> MAIRLYKLAVALGVFIVSAPAFSHGHHSHGKPLTEVEQKAANGVFDDANVQNRTLSDWDGVWQSVYPLLQSGKLDPVFQKKADADKTKTFAEIKDYYHKGYATDIEMIGIEDGIVEFHRNNETTSCKYDYDGYKILTYKSGKKGVRYLFECKDPESKAPKYIQFSDHIIAPRKSSHFHIFMGNDSQQSLLNEMENWPTYYPYQLSSEEVVEE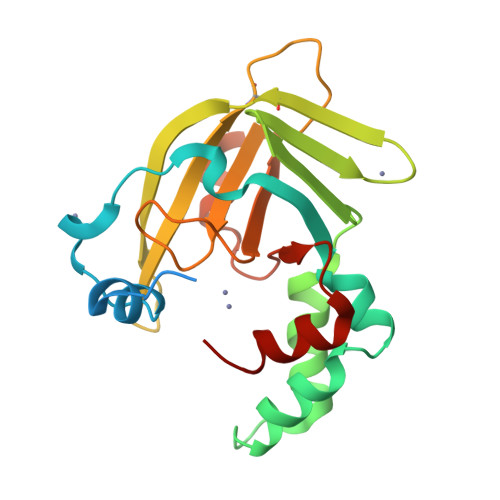MMSH>GRIVWDGSFNNYTTPADFDRWSWANQVGTYQWYIKGSGPTSRYLNLDPSYKNPAITSELRGLKVTIDTTATWNSQMMRTELIPQTNANLGQGNLFYHFSIKRTNTNAPDPTLEHQVMFFESHFTELKYGVGSNPSNLGWYAGGTERWSTP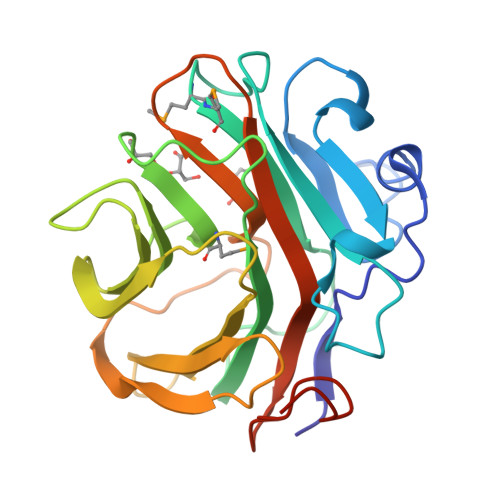FTADTWFNFAYDIDFTAKTVGLWASTNGNPLVKVVQNVPANTFTDSRDFHVGVLRIVNRNPPEDWYVSGVYIEEGPITTQIGDGAAALEHHHHHH[4x]> MERREEQPGAAGAGAAPALDFTVENVEKALHQLYYDPNIENKNLAQKWLMQAQVSPQAWHFSWQLLQPDKVPEIQYFGASALHIKISRYWSDIPTDQYESLKAQLFTQITRFASGSKIVLTRLCVALASLALSMMPDAWPCAVADMVRLFQAEDSPVDGQGRCLALLELLTVLPEEFQTSRLPQYRKGLVRTSLAVECGAVFPLLEQLLQQPSSPSCVRQKVLKCFSSWVQLEVPLQDCEALIQAAFAALQD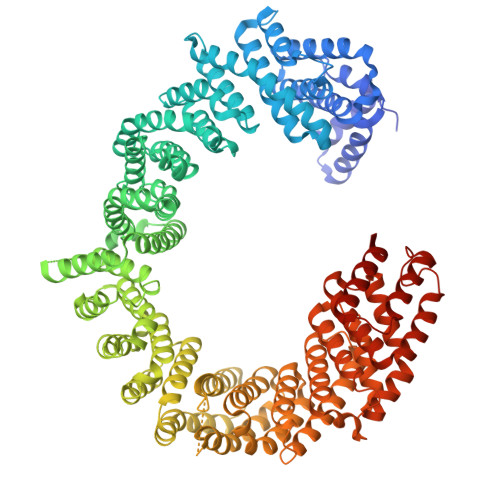SELFDSSVEAIVNAISQPDAQRYVNTLLKLIPLVLGLQEQLRQAVQNGDMETSHGICRIAVALGENHSRALLDQVEHWQSFLALVNMIMFCTGIPGHYPVNETTSSLTLTFWYTLQDDILSFEAEKQAVYQQVYRPVYFQLVDVLLHKAQFPSDEEYGFWSSDEKEQFRIYRVDISDTLMYVYEMLGAELLSNLYDKLGRLLTSSEEPYSWQHTEALLYGFQSIAETIDVNYSDVVPGLIGLIPRISISNVQLADTVMFTIGALSEWLADHPVMINSVLPLVLHALGNPELSVSSVSTLKKICRECKYDLPPYAANIVAVSQDVLMKQIHKTSQCMWLMQALGFLLSALQVEEILKNLHSLISPYIQQLEKLAEEIPNPSNKLAIVHILGLLSNLFTTLDISHHEDDHEGPELRKLPVPQGPNPVVVVLQQVFQLIQKVLSKWLNDAQVVEAVCAIFEKSVKTLLDDFAPMVPQLCEMLGRMYSTIPQASALDLTRQLVHIFAHEPAHFPPIEALFLLVTSVTLTLFQQGPRDHPDIVDSFMQLLAQALKRKPDLFLCERLDVKAVFQCAVLALKFPEAPTVKASCGFFTELLPRCGEVESVGKVVQEDGRMLLIAVLEAIGGQASRSLMDCFADILFALNKHCFSLLSMWIKEALQPPGFPSARLSPEQKDTFSQQILRERVNKRRVKEMVKEFTLLCRGLHGTDYTADY> GCCCGCACAAGCGGUGGAGCAUGUGGUUUAAUUCGAUGCAACGCGAAGAACCUUAC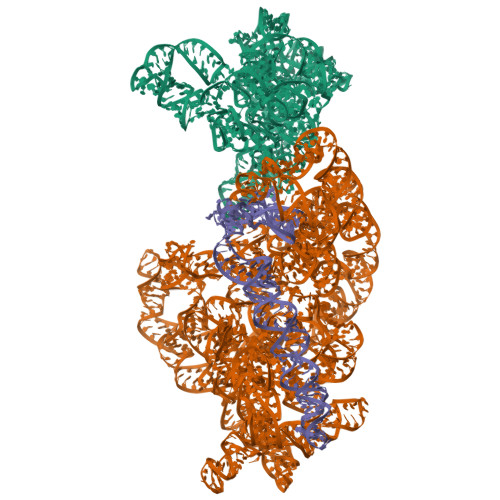CUGGUCUUGACAUCCACGGAAGUUUUCAGAGAUGAGAAUGUGCCUUCGGGAACCGUGAGACAGGUGCUGCAUGGCUGUCGUCAGCUCGUGUUGUGAAAUGUUGGGUUAAGUCCCGCAACGAGCGCAACCCUUAUCCUUUGUUGCCAGCGGUCCGGCCGGGAACUCAAAGGAGACUGCCAGUGAUAAACUGGAGGAAGGUGGGGAUGACGUCAAGUCAUCAUGGCCCUUACGACCAGGGCUACACACGUGCUACAAUGGCGCAUACAAAGAGAAGCGACCUCGCGAGAGCAAGCGGACCUCAUAAAGUGCGUCGUAGUCCGGAUUGGAGUCUGCAACUCGACUCCAUGAAGUCGGAAUCGCUAGUAAUCGUGGAUCAGAAUGCCACGGUGAAUACGUUCCCGGGCCU;> AAUUGAAGAGUUUGAUCAUGGCUCAGAUUGAACGCUGGCGGCAGGCCUAACACAUGCAAGUCGAACGGUAACAGGAAGAAGCUUGCUUCUUUGCUGACGAGUGGCGGACGGGUGAGUAAUGUCUGGGAAACUGCCUGAUGGAGGGGGAUAACUACUGGAAACGGUAGCUAAUACCGCAUAACGUCGCAAGACCAAAGAGGGGGACCUUCGGGCCUCUUGCCAUCGGAUGUGCCCAGAUGGGAUUAGCUAGUAGGUGGGGUAACGGCUCACCUAGGCGACGAUCCCUAGCUGGUCUGAGAGGAUGACCAGCCACACUGGAACUGAGACACGGUCCAGACUCCUACGGGAGGCAGCAGUGGGGAAUAUUGCACAAUGGGCGCAAGCCUGAUGCAGCCAUGCCGCGUGUAUGAAGAAGGCCUUCGGGUUGUAAAGUACUUUCAGCGGGGAGGAAGGGAGUAAAGUUAAUACCUUUGCUCAUUGACGUUACCCGCAGAAGAAGCACCGGCUAACUCCGUGCCAGCAGCCGCGGUAAUACGGAGGGUGCAAGCGUUAAUCGGAAUUACUGGGCGUAAAGCGCACGCAGGCGGUUUGUUAAGUCAGAUGUGAAAUCCCCGGGCUCAACCUGGGAACUGCAUCUGAUACUGGCAAGCUUGAGUCUCGUAGAGGGGGGUAGAAUUCCAGGUGUAGCGGUGAAAUGCGUAGAGAUCUGGAGGAAUACCGGUGGCGAAGGCGGCCCCCUGGACGAAGACUGACGCUCAGGUGCGAAAGCGUGGGGAGCAAACAGGAUUAGAUACCCUGGUAGUCCACGCCGUAAACGAUGUCGACUUGGAGGUUGUGCCCUUGAGGCGUGGCUUCCGGAGCUAACGCGUUAAGUCGACCGCCUGGGGAGUACGGCCGCAAGGUUAAAACUCAAAUGAAUUGACGGGG;> UGUACACACCGCCCGUCACACCAUGGGAGUGGGUUGCAAAAGAAGUAGGUAGCUUAACCUUCGGGAGGGCGCUUACCACUUUGUGAUUCAUGACUGGGGUGAAGUCGUAACAAGGUAACCGUAGGGGAACCUGCGGUUGGAUCA(S)-2-AMINO-5-(2-HYDROXYACETIMIDAMIDO)PENTANOIC ACID | C7 H15 N3 O3 | 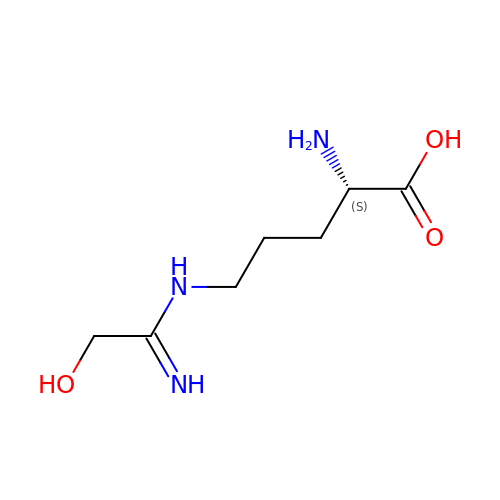TXBVSXZGQDGYCU-YFKPBYRVSA-N> GSDGDQC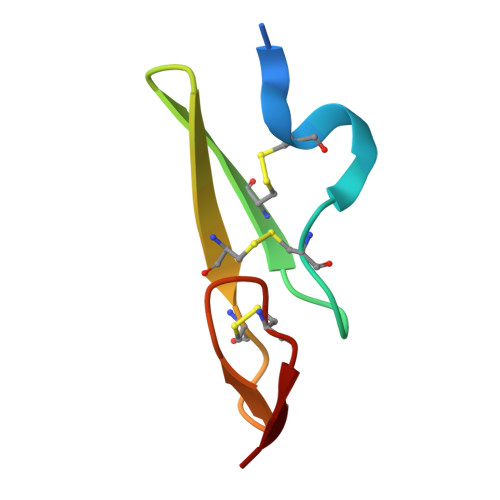ASSPCQNGGSCKDQLQSYICFCLPAFEGRNCETHK>[15x]MNKRHALLLTAVLGMATAYAQTAPTTTTVNTLQTVYRDPSLTSAPITANVGKYVGPLSTFLASIAKSAGYEVVFNFNIDALALINGEIVFGNSTASVTTSYATPLGRPQELPAKPVVHNFSNAPFNEAWPLLMDVYELDYQLVKVGSANVIRIGQRPKQLALPLKFISAESALTAIEKFFGEEKFETVISLDSNNKPFQTTRPTGKFGLPNSIKVIPDSSNKRLIIGSNSEDGIRIRSFVETIDVQSSGKVISTDSISEIYIVRGQKESVLQFLRDSFPELIVTDYASGGLAIEGPRTSVNRAIILLGQVDRAPEIPIVQRIYTVRGQAADITALLAAQYPTLRVTPVGQTGQLVLNGAQAQLDTALALLEQVDRPAPVAESRTVQRVF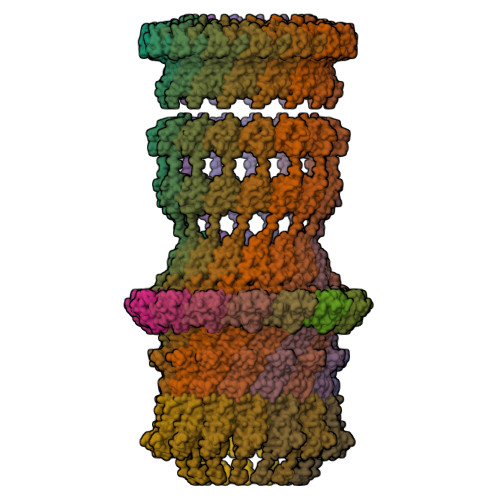QLVNASAEEVKATLEGTLARDLTADSNNDVLPNVPVTATDANGNTTVVSVPNALGKTANQGTANAQAQTAQTPANTQQATLIADKRTNSLIVRGTPEQVAQVAELVPQLDQVVPQINVQVRIQEVNERALQSLGLNWRATFGGFNVAVSGGTGLAATFNPTQSFLGFNIFPTLTALETQGLTRRVYDGNVTMQSGQRSLSATGGAQNASSGAAASVKSGGRLEINIPSAAGNIVRQIDYGLNLDFFSPQVAPDGTITLRIRGQVNQPATAITADSLPNLIDFTNSEAQSTITFKNGQTILMSGLLGSTETTNRSGVPFLSSLPGVGAAFGEKRTEKTQSQLLVIITGTVVK;>MTALGVEHDQHPACGGGSLTRHLQLIRLPGGGLSMLRFFCASLLLTGLLASCTPRVTTVAGVTVTPVLIKVSEGAAPGDTLTIQGRYLGNAQTARVIIGADENGQGGTAFPASAVQSWSDTEIVLKVPEGMPAGGSWLFVEVGGKRSTGLRVSVR[15x];>[15x]MTMKKMFPVLLLGGLLLAGCGTVGLGSGRVNVGVDVGDAGSEQVATLTITPEKCDDKGVCTPQKQELSITDGQPVTFTFTARPGSEAVTIEGYRVLSDRLDGVERADPKNPVENAKMNLYVPSGYACEGLTAGASCQGNESDIRIANGQPVQHQIYFASGLGARAAAKGANVTRVVDLEFYGFSANNVPFTRKVTGIVSQGSYVVKTN>[4x]GPHMMSGEKRVLSGRVAVVTGSRKGIGLGIAMRLAMAGADVVLNGRRQSPEDSAIVEKVAAYGTRVRCFAANMKDRAQVEALIKFTEKELGAVEILVNNAGIQHVSPVETFPSDKWDEIIALNLTSAFHATQLCLPSMRQRGWGRIINIASVQGLVGSMNKSAYCAAKHGLIGFTKVVALETATTGITCN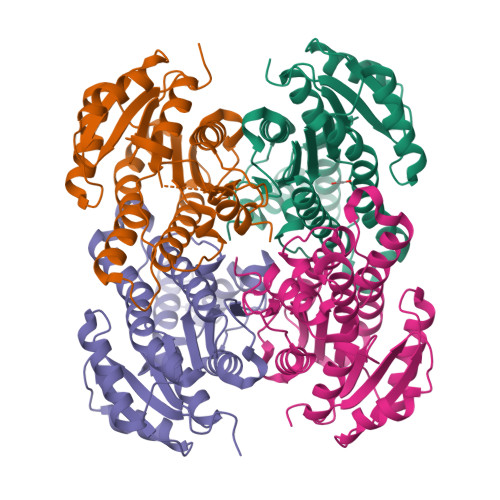AICPGYVYTPLVEEQIKAVAEAKYGGDMEAATQAFLCEKQPAKAFVTVEQVGDAAVFLASPGADMIRGTTITVDGGWVAQ>[3x]MAMNKQNNYSDDSIQVLEGLEAVRKRPGMYIGS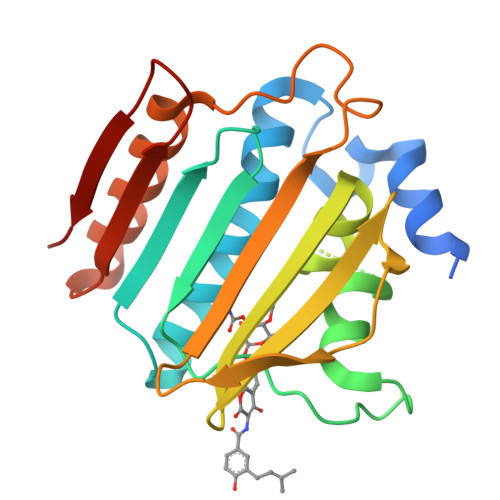TDKRGLHHLVYEIVDNSVDEVLNGYGNEIDVTINKDGSISIEDNGRGMPTGIHKSGKPTVEVIFTVLHAGGKFGQGGYKTSGGLHGVGASVVNALSEWLEVEIHRDGNIYHQSFKNGGSPSSGLVKKGKTKKTGTKVTFKPDDTIFKASTSFNFDVLSERLQESAFLLKNLKITLNDLRSGKERQEHYHYEE N-[(2S,4S)-1-({4-[2-(3,5-dimethyl-1,2-oxazol-4-yl)ethyl]piperidin-1-yl}sulfonyl)-4-(5-fluoropyrimidin-2-yl)-2-methylpentan-2-yl]-N-hydroxyformamide | C23 H34 F N5 O5 S | 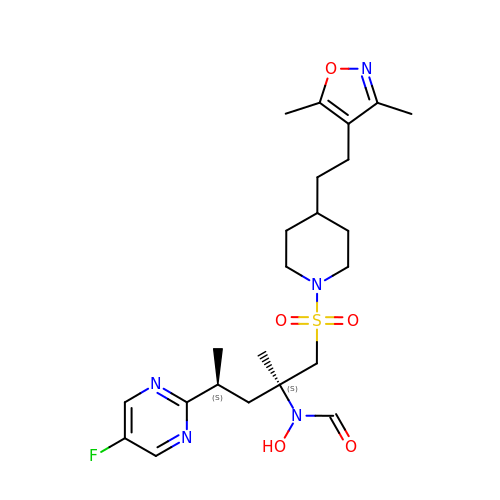UAGAABCJKYADIR-HJPURHCSSA-N(1S)-1-CARBOXY-5-[(3-CARBOXYPROPANOYL)AMINO]-8,9-DIHYDROXY-1,2,3,4-TETRAHYDROPYRIMIDO[1,2-A]QUINOLIN-11-IUM | C17 H18 N3 O7 | 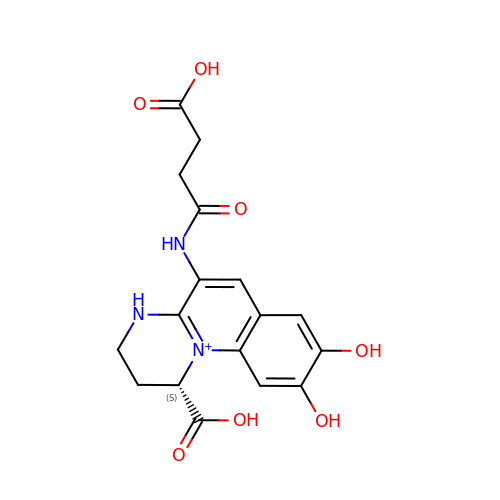PKIXPGNFUHEBHN-JTQLQIEISA-O N-[(1S,2R)-3-{[1-(3-tert-butylphenyl)cyclohexyl]amino}-1-(3,5-difluorobenzyl)-2-hydroxypropyl]acetamide 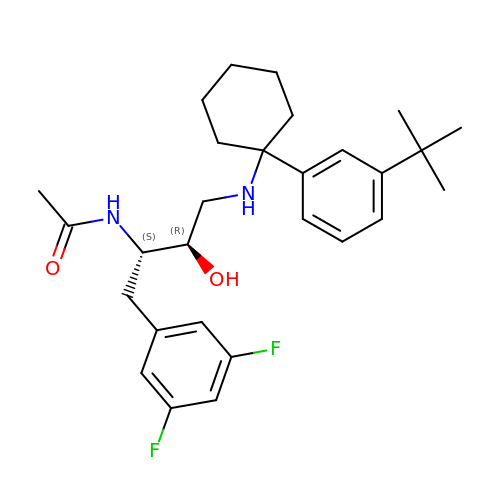| C28 H38 F2 N2 O2 | RJXIEHBFRZLGTH-IZZNHLLZSA-N>SLTMDVPPTIHVPLPPTSYPAFDAAIFTDIGGRKHQEDRFTLCPQLVPGRDDCAFFGVFDGTVGDFASENVKDLVVPQLISSPAWQEVTEMLRSDVPATEVDEKLPQLLDQAVDDMYKNADNELVKMCEQLNKDYASSTSVTAVLAKGFVAVGHLGDSRIAMGVETPNGLNCEFLTVDHKPDMPHEKLRIMRNGGSVEYLHNHNNKPFIRGGDFSFRKSRGEQPMQLQYSRAFGGKDLKMYGLSNQPDVRVVRVTPQHRVMILATDGLW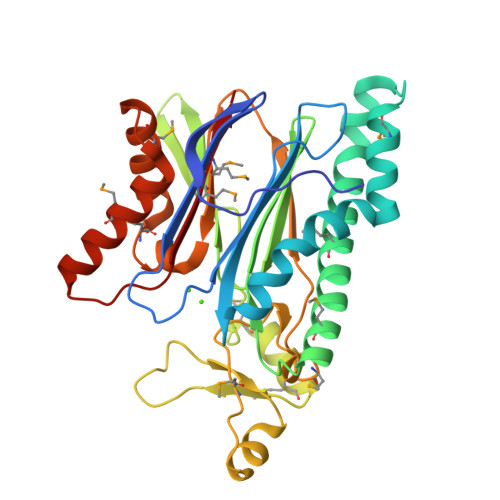DVMSAAQAVEIAMQARQEGRNPAQALVEMTLAEQQSRNQSADNITAMTVFFKKTD[3x]>MEEPEEPADSGQSLVPVYIYSPEYVSMCDSLAKIPKRASMVHSLIEAYALHKQMRIVKPKVASMEEMATFHTDAYLQHLQKVSQEGDDDHPDSIEYGLGYDCPATEGIFDYAAAIGGATITAAQCLIDGMCKVAINWSGGWHHAKKDEASGFFYLNDAVLGILRLRRKFERILYVDLDLHHGDGVEDAFSFTSKVMTVSLHKFSPGFFPGTGDVSDVGLGKGRYYSVNVPIQDGIQDEKYYQICESVLKEVYQAFNPKAVVLQLGA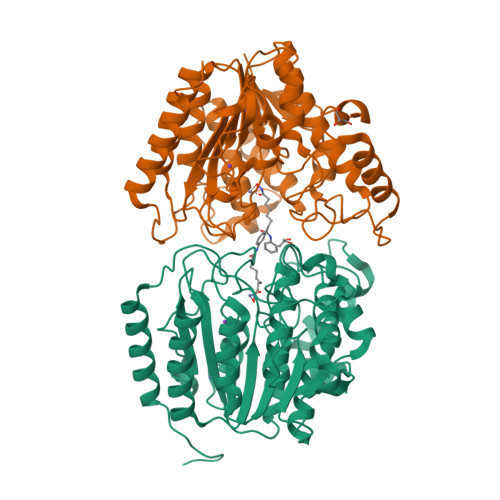DTIAGDPMCSFNMTPVGIGKCLKYILQWQLATLILGGGGYNLANTARCWTYLTGVILGKTLSSEIPDHEFFTAYGPDYVLEITPSCRPDRNEPHRIQQILNYIKGNLKHVVIEGRGSHHHHHH[2x]> MENTENSVDSKSIKNLEPKIIHGSESMDSGISLDNSYKMDYPEMGLCIIINNKNFHKSTGMTSRSGTDVDAANLRETFRNLKYEVRNKNDLTREEIVELMRDVSKEDHSKRSSFVCVLLSHGEEGIIFGTNGPVDLKKITNFFRGDRCRYLTGKPKLFIIQACRGTELDCGIETD;> SGVDDD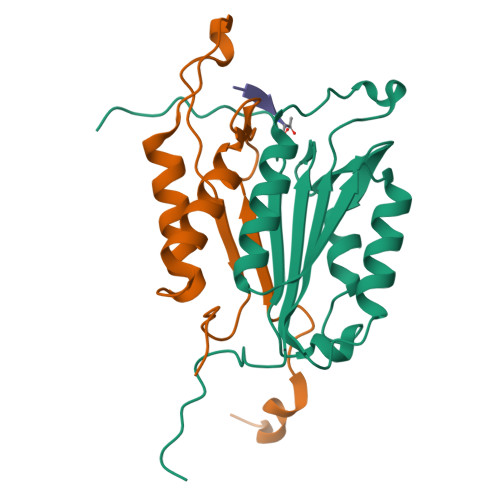MACHKIPVEADFLYAYSTAPGYYSWRNSKDGSWFIQSLCAMLKQYADKLEFMHILTRVNRKVATEFESFSFDATFHAKKQIPCIVSMLTKELYFYHH> MNFKIKAKGHKNVLSLHKSTFEITKDKDLSLSGDCIIGLDIDKCMLDFPKEFKEKLANDETIVTVKLKSPNAYDEIVGYGHHDLTLDHPTDIVCRK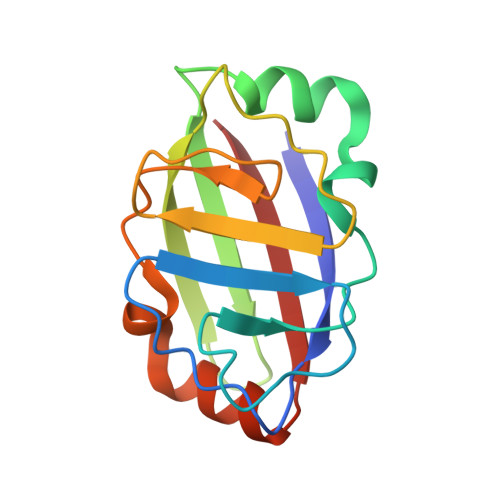SDFICSRTLMIKSDKAAIDLNRDLIEDLANGESLDVEIILS>MVLGYVSDMHTELASISQLVIAKIETIDNDILNKDIVNFIMCRSNLDNPFISFLDTVYTIIDQENYQTELINSLDDNEIIDCIVNKFMSFYKDNLENIVDAIITLKYIM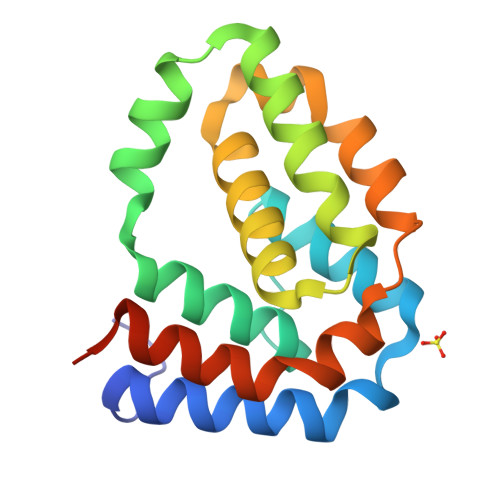NNPDFKTTYAEVLGSRIADIDIKQVIRENILQLSNDIRERYLGSKHHHHHH[8x]>[2x]KHS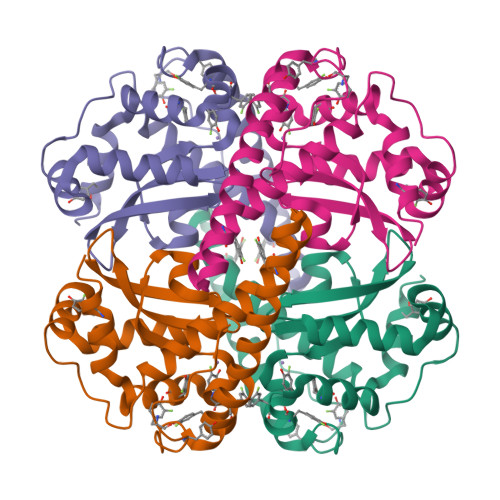LPDLPYDYGALEPHINAQIMQLHHSKHHAAFVNNLNVTEEKYQEALAKGDVTAQIALQPALKFNGGGHINHSIFWTNLSPNGGGEPKGELLEAIKRDFGSFDKFKEKLTAASVGVQGSGWGWLGFNKERGHLQIAACPNQDPLQGTTGLIPLLGIDVWEHAYYLQYKNVRPDYLKAIWNVINWENVTERYMACKK>MELALQRVRDIMIPRSQMITLKRNQTLDECLDVIIESAHSRFPVISEDKDHIEGILMAKDLLPFMRSDAEAFSMDKVLRQAVVVPESKRVDRMLKEFRSQRYHMAIVIDEFGGVSGLVTIEDILELIVG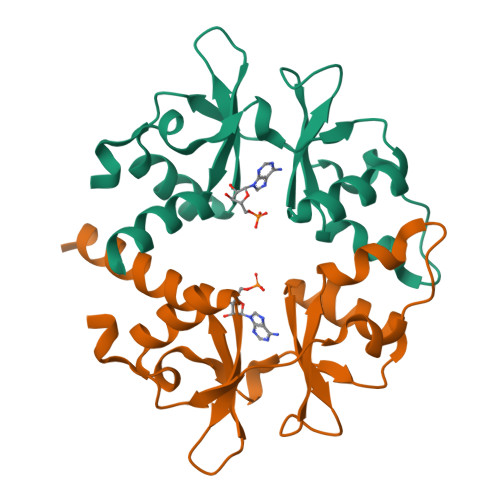EIEKGQFLEHHHHHH[2x]>[4x]HHHHHHDSGLVPRGSHMHGNHTHWGYTGHDSPESWGNLSEEFRLCSTGKNQSPVNITETVSGKLPAIKVNYKPSMVDVENNGHTIQVNYPEGGNTLTVNG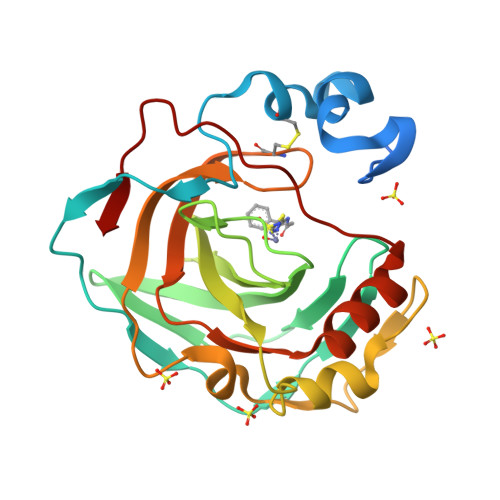RTYTLKQFHFHVPSENQIKGRTFPMEAHFVHLDENKQPLVLAVLYEAGKTNGRLSSIWNVMPMTAGKVKLNQPFDASTLLPKRLKYYRFAGSLTTPPCTEGVSWLVLKTYDHIDQAQAEKFTRAVGSENNRPVQPLNARVVIE L-GAMMA-GLUTAMYL-S-[(2S)-2-HYDROXY-2-PHENYLETHYL]-L-CYSTEINYLGLYCINE | C18 H25 N3 O7 S | 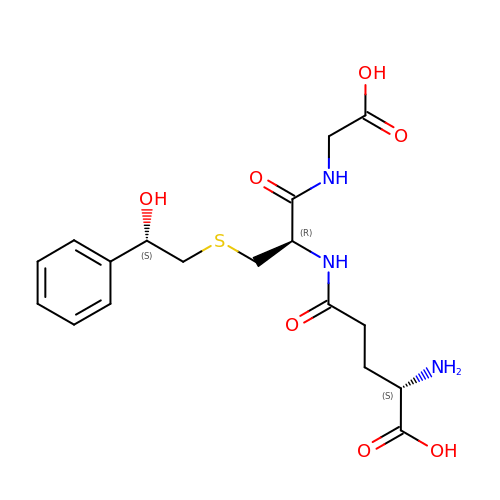SZOWFFWYTHGUAW-MELADBBJSA-N> MTEFWLISAPGEKTCQQTWEKLHAATTKNNNLAVSSKFNIPDLKVG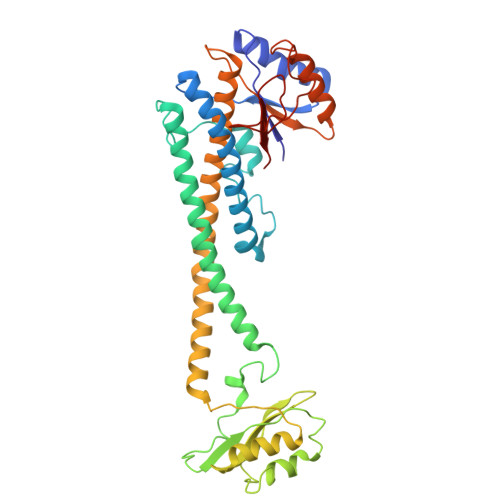TLDVLVGLSDELAKLDAFVEGVVKKVAQYMADVLEDSKDKVQENLLASGVDLVTYITRFQWDMAKYPIKQSLKNISEIIAKGVTQIDNDLKSRASAYNNLKGNLQNLERKNAGSLLTRSLAEIVKKDDFVLDSEYLVTLLVVVPKLNHNDWIKQYETLAEMVVPRSSNVLSEDQDSYLCNVTLFKKAVDDFRHKARENKFIVRDFQYNEEEMRADKEEMNRLSTDKKKQFGPLVRWLKVNFSEAFIAWIHIKALRVFVESVLRYGLPVNFQAMLLQPNKKSVKKLREVLHELYKHLDSSAAAIIDAPMDIPGLNLSQQEYYPYVYYKIDCNLLEFK>SNAMNTGEMKINWVSRYMPLLNKIAEEYSREKPLSGFTVGMSIHLEAKTAYLAITLSKLGAKVVITGSNPLSTQDDVAEALRSKGITVYARRTHDESIYRENLMKVLDERPDFIIDDGGDLTVISHTEREEVLENLKGVSEETTTGVRRLKALEETGKLRVPVIAVNDSKMKYLFDNRYGTGQSTWDAIMRNTNLLVAGKNVVVAGYGWCGRGIALRAAGLGARVIVTEVDPVKAVEAIMDGFTVMPMKEAVKIADFVITASGNTDVLSKEDILSLKDGAVLANAGHFNVEIPVRVLEEIAVEKFEARPNVTGYTLENGKTVFLLAEGRLVNLAAGDGHPVEIMDLSFALQIFAVLYLLENHRKMSPKVYMLPDEIDE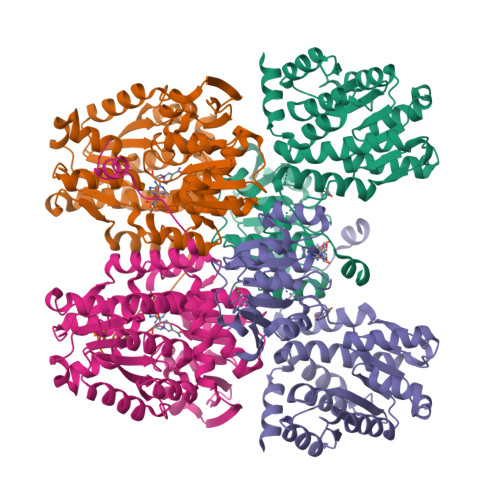RVARMKLDSLGVKIDELTEKQRRYLRSWQ[2x]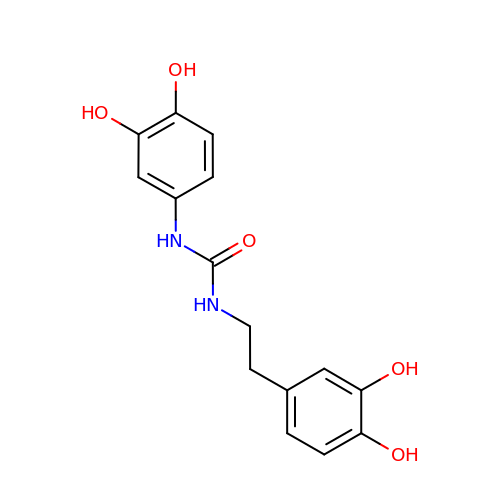N-(3,4-dihydroxyphenyl)-N'-[2-(3,4-dihydroxyphenyl)ethyl]urea | C15 H16 N2 O5 | XPAUTCCLOUPUGJ-UHFFFAOYSA-N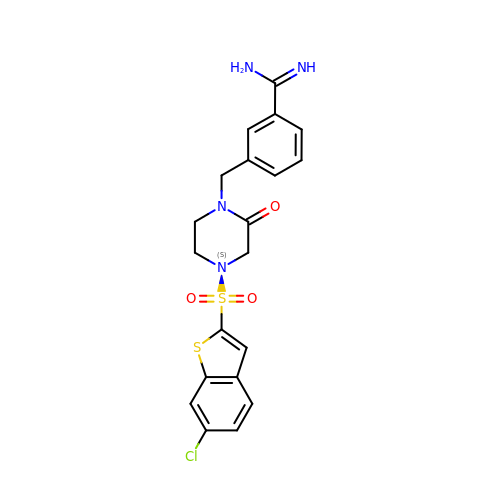3-({4-[(6-CHLORO-1-BENZOTHIEN-2-YL)SULFONYL]-2-OXOPIPERAZIN-1-YL}METHYL)BENZENECARBOXIMIDAMIDE | C20 H19 Cl N4 O3 S2 | PRMSFVUWLBPPLY-UHFFFAOYSA-N> MESPATQVDPANSPLEPYHIYPEAKSCPVAKVGLWNGTPAHVFSGYE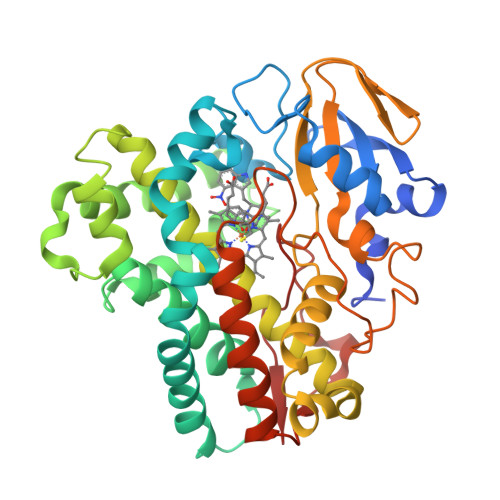DVRTVLQDRRFSSDSRRPNFTELTPTLQSQAAAPPFVRTDNPDHRRLRGTIAREFLPKHIELLRPAIREIVQGVLDGLAETAPPQDMLEAFAVPVASATVFRLLGIPAEDRALLTRCVKGVVSAVGSEDEGAEVFRTLGEYIGGLVQDPSELPEDSLIRRLVTGPYQEKQLTFHETIGVILMLIVGGYDTTASTISLSLVSYALQPEKFSVVHEHPERIPLLVEELLRYHTVSQLGLGRIATEDVEVGGVTVRAGQMVVAALPLANRDESVFPNPDELDFDRPSVPHVGFGYGPHQCVGQALARVELQEAIPAVIRRLPGMRLACALEDLPFRHDMATYGIHELPMTW>[6x]MAHHHHHHMAKTGASKVIKGGTVITADRTFRADILIEDGKIAAIGDSLEGDEVIDASGCYVMPGGIDPHTHLQMPFMGTYSSDDFDTGTAAALAGGTTMVVDFVLPDSEGNLLDALQEWFQKAGKARTDYSFHMAITGWNERTFNEMAEVVKRGINTFKHFMAYKGALMVNDDEMFASFQRCAELGAMPLVHAENGDIVAQLQAKL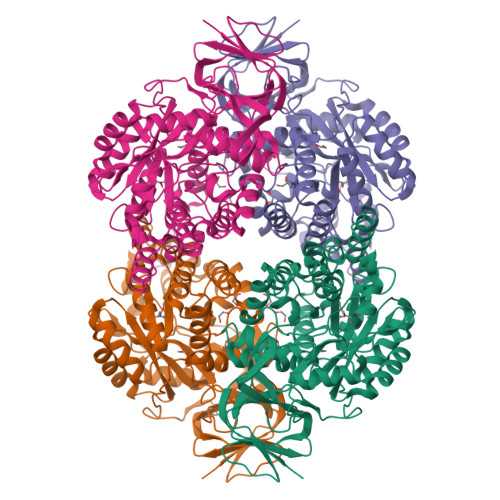MAEGNDGPEAHAYSRPPEVEGEATNRAIMIADQAGVPLYVVHVSCEQSHEAIRRARQKGMRVFGEPLIQHLTLDESEYHNRDWDYAARRVMSPPFRDKLNQDSLWAGLAAGSLQCVATDHCAFTTEQKRYGIGNFTKIPNGTGGLEERMPVLWTRGVRTGRLTPNEFVAVTSTNIAKILNIYPQKGAVVPGADADLVIWDPETTKKISAKTQHSSIDYNVFEGFELKGLPIMTLSRGRIAFDKGQVTAKPGDGRFIEREPNGAVNRALSQWKEIVAPRKVERSAEHMPIGV> IPEYVDWRQKGAVTPVKNQGSCGSCWAFSAVVTIEGIIKIRTGNLNQYSEQELLDCDRRSYGCNGGYPWSALQLVAQYGIHYRNTYPYEGVQRYCRSREKGPYAAKTDGVRQVQPYNEGALLYSIANQPVSVVLEAAGKDFQLYRGG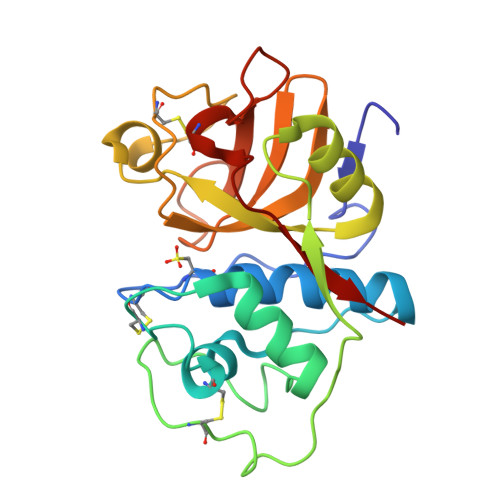IFVGPCGNKVDHAVAAVGYGPNYILIKNSWGTGWGENGYIRIKRGTGNSYGVCGLYTSSFYPVKN TRIFLUOROFURNESYL DIPHOSPHATE | C15 H25 F3 O7 P2 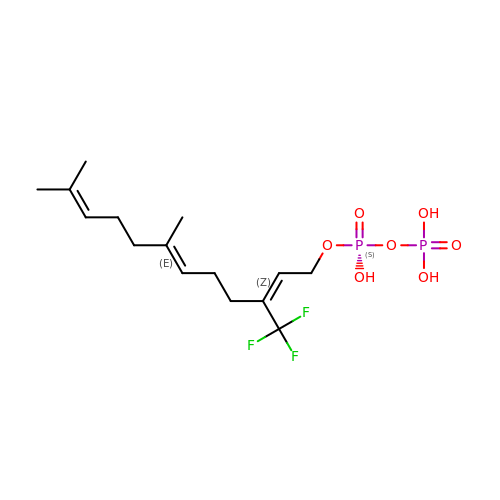| PXLMLAFPAPGGKK-GVCYOOEQSA-N>MNLEKINELTAQDMAGVNAAILEQLNSDVQLINQLGYYIVSGGGKRIRPMIAVLAARAVGYEGNAHVTIAALIEFIHTATLLHDDVVDESDMRRGKATANAAFGNAASVLVGDFIYTRAFQMMTSLGSLKVLEVMSEAVNVIAEGEVLQLMNVNDPDITEENYMRVIYSKTARLFEAAAQCSGILAGCTPEEEKGLQDYGRYLGTAFQLIDDLLDYNADGEQLGKNVGDDLNEGKPTLPLLHAMHHGTPEQAQMIRTAIEQ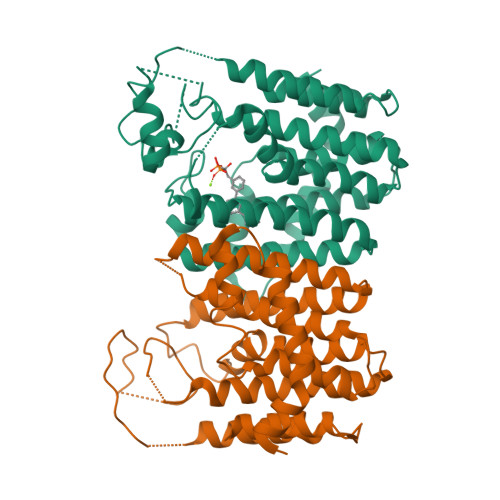GNGRHLLEPVLEAMNACGSLEWTRQRAEEEADKAIAALQVLPDTPWREALIGLAHIAVQRDR[4x]Dehydroquinate dehydratase (DHQD) catalyzes the conversion of 3-dehydroquinic acid (DHQ) into 3-dehydroshikimic acid in the mid stage of the shikimate pathway, which is essential for the biosynthesis of aromatic amino acids and folates. Here, we report two the crystal structures of type II DHQD (CgDHQD) derived from Corynebacterium glutamicum, which is a widely used industrial platform organism. The enzyme forms a homododecamer consisting of four trimers with three interfacial active sites. Our analysis revealed that the monomer is composed of repetitive α/β domains, forming a flavodoxin fold with central parallel β sheets arranged in a specific order.

We determined the structures for CgDHQDWT with the citrate at a resolution of 1.80Å and CgDHQDR19A with DHQ complexed forms at a resolution of 2.00 Å, respectively. The asymmetric unit of the citrate- and DHQ-bound structures contained four and six molecules, respectively, highly homologous with alpha carbon, with root mean square deviation values within 0.2. The DHQ-bound structure of CgDHQD explained the substrate-binding mode of the enzyme. The substrate is stabilized by hydrogen bonds with a water molecule, side chains of N75, H81, D88, H101, S103, and R112, and main chains of I102 and S103. Moreover, the neighboring residues L13, G77, G78, T80, and P105 organize the substrate-surrounding environment of the active site. A glycerol molecule exists in this structure to occupy the space of R19A variation that eliminates the enzyme activity for crystallographic benefit. There are six residues that directly participate in enzyme catalysis, including R19, Y24, N12, E99, H101, and R108. The Y24 positions toward the 2-carbon of DHQ to function as a general base catalyst with R19 and R108 activators. The position of the water molecule is known to be crucial, and it mediates the initial electron transfer from Y24 to N12. H101 and E99 give a proton to the leaving 1-hydroxyl group of DHQ.

>[6x]MPGKILLLNGPNLNMLGKAEPDIYGHDTLEDVVALATAEAAKHGLEVEALQSNHEGELIDALHNARGTHIGCVINPGGLTHTSVALLDAVKASELPTVEVHISNPHAREEFRHHSYISLAAVSVIAGAGIQGYRFAVDILANLKKLEHHHHHH>MKETILVNLVSEQTIPNVQFIKWYFNKKQTPMKILLVSTKEMEQKEKSLFIKNALHFSDSFVEWETIHTDGNDISKTENILTDYFRDNEYKNIIVNITGGTKIMSLAAFDFFNNKPNTEIFYQPIGKELQELYPNKQKYDMFEVLSLKEYLDAHGISYKYDNECVKDWNYNKTVYDLCVADNRELIKGMIALQNNSYFNNVYKRKDFLDFTQIEEEKFIAINHPAATKENMIKILQIFGFDVSRIEHKHIRYITGGWFEEYVYQKICNEYHNVDEKNVALNVTIQKGNDKNELDVIYLDKDNKLHVIECKSFVDGNEGNRVLNDALYKLQAIIKSKFGLYVKQHLYTKSIIEKETPLNRAKEFGIDIKDGTQLGSG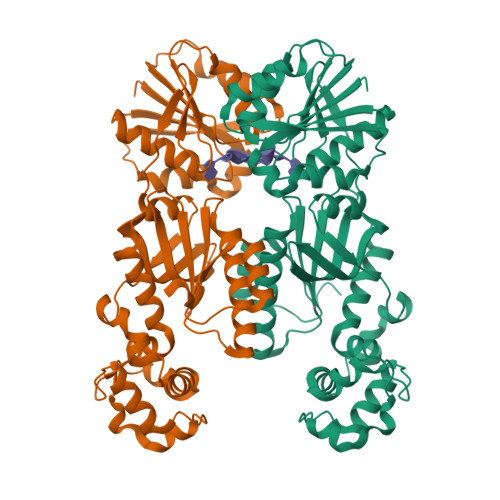HHHHHH[4x]> GASHPEIEKAQREIIEA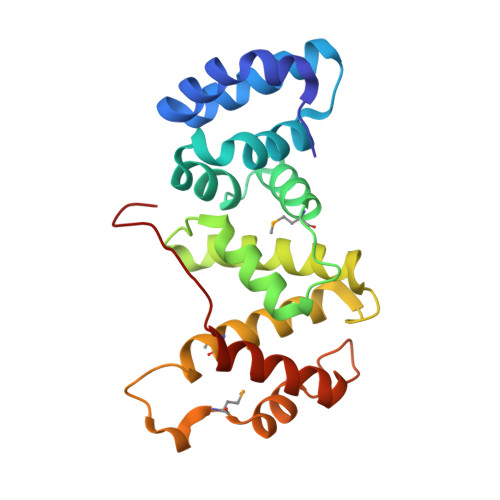FNAKPKNGINKIKEICEQYKISPNEEIAEFFHQQRKNLDLEAVGDYLSSPEAENQQVLKAFTSQMNFNGQSFVEGLRTFLKTFKLPGEAQKIDRLVQSFSGAYFQQNPDVVSNADAAYLLAFQTIMLNTDLHNPSIPEKNKMTVDGLKRNLRGGNNGGDFDAKFLEELYSEIKAKPFELNFVKTSP>[6x]MHHHHHHLQTAEAPWSQAETQSAHALFRKAYQRELDGLL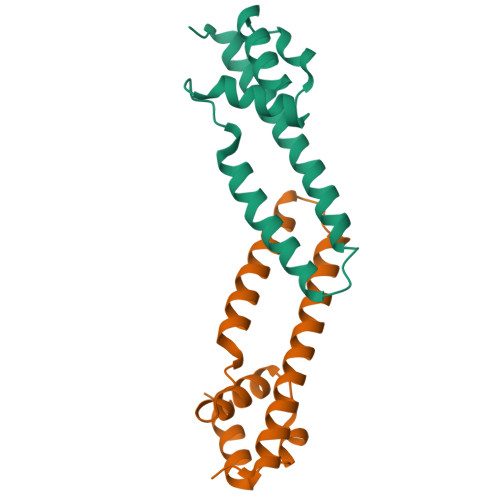ATVQAQASQITQIDDLWKLHDFLSAKKHEIDGKYDDRQSVIIFVFAQLLKEGLVQAEELTFLAADKQSKIKALARL>GGDGSYVSVPSPLGKIKSMTKEKADILLLRAGLPSHFHLQLSEIEFHEIIGSGSFGKVYKGRCRNKIVAIKRYRANTYCSKSDVDMFCREVSILCQLNHPCVIQFVGACLNDPSQFAIVTQYISGGSLFSLLHEQKRILDLQSKLIIAVDVAKGMEYLHN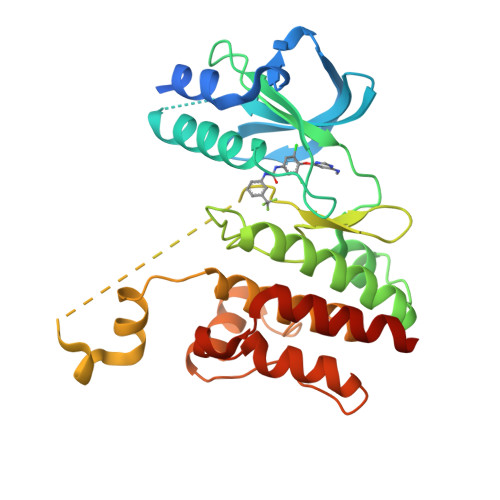LTQPIIHRDLNSHNILLYEDGHAVVADFGESRFLQSLDEDNMTKQPGNLRWMAPEVFTQCTRYTIKADVFSYALCLWEILTGEIPFAHLKPAAAAADMAYHHIRPPIGYSIPKPISSLLIRGWNACPEGRPEFSEVVMKLEECLCNIELMS[4x]>MMVSFTARAKSNVMAYRLLAYSQGDDIIEISHAAENTIPDYVAVKDVDKGDLTQVNMYPLAAWQVIAGSDIKVGDNLTTGKDGTAVPTDDPSTVFGYAVEEAQEGQLVTLVISRSKLEH[6x]

The bacteriophage ϕ29, a representative of bacteriophages with a short non-contractile tail, has an ~19 kb dsDNA genome encoding ~20 proteins. Both 5ʹ ends of the genome are covalently connected to the terminal protein gene product 3 (gp3). ϕ29 infects the Gram-positive Bacillus subtilis cells by injecting the genome–gp3 complex into the host-cell cytoplasm using a short non-contractile tail, leaving the genome emptied virion on the cell surface. Here, we report the cryo-electron microscopy (cryo-EM) structural studies of the ϕ29 prohead, the mature and the genome-emptied virions at near-atomic resolutions up to 3.2 Å. Our results show structural details of the complex capsid, the DNA packaging motor and the entire tail machinery, and provide a molecular basis for understanding the assembly, maturation and infection mechanisms of the bacteriophage ϕ29.

Each of the head fibers is a homotrimer of gp8.516,19, which consists of a pseudo-hexagonal base and a protruding stem with a unique three-stranded helix-turn-helix supercoil structure. We also determined the crystal structure of the N-terminal pseudo-hexagonal base (gp8.5 N-base, residues 1–116) to a resolution of 1.8 Å by molecular replacement using the EM map as a search model. The crystal structure shows a similar homotrimer with a β-strand missing from each gp8.5-N-βA domain of the trimer. The results showed that the N-terminal 110 residues of gp8.5 form two small β-barrel domains (gp8.5-N-βA and N-βB) connected by a short linker (residues 58–61). The two small β-barrel domains are similar to each other. The monomers in the trimer are associated with each other through hydrophobic interactions and have large buried surfaces in between them. The head fibers at the quasi-3-fold positions can further stabilize the capsid.> SSADKERLARENHSEIERRRRNKMTAYITELSDMVPTCSALARKPDKLTILRMAVSHMKSLRGTGNTSTDGSYKPSFLTDQELKHLILEAADGFLFIVSCETGRVVYVSDSVTPVLNQPQSEWFGSTLYDQVHPDDVD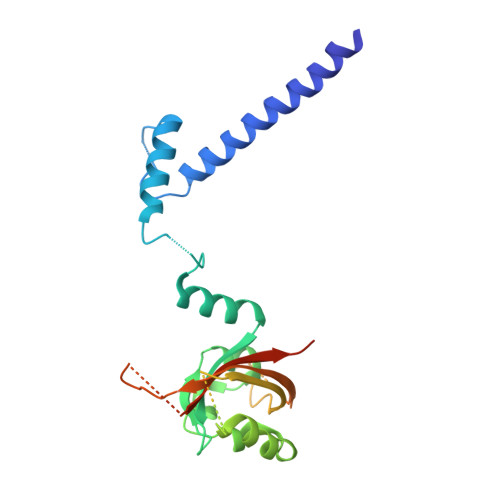KLREQLSTSENALTGRVLDLKTGTVKKEGQQSSMRMCMGSRRSFICRMRCGTSSVDPVSMNRLSFLRNRCRNGLGSVKEGEPHFVVVHCTGYIKAWPPAGVSLPDDDPEAGQGSKFCLVAIGRLQVTSSPNCTDMSNICQP> MLTEGISIQSYDGHTFGALVGSPAKAPAPVIVIAQDIFGVNAFMRETVSWLVDQGYAAVCPDLYARQAPGTALDPQDERQREQAYKLWQAFDMEAGVGDLEAAIRYARHQPYSNGKVGLVG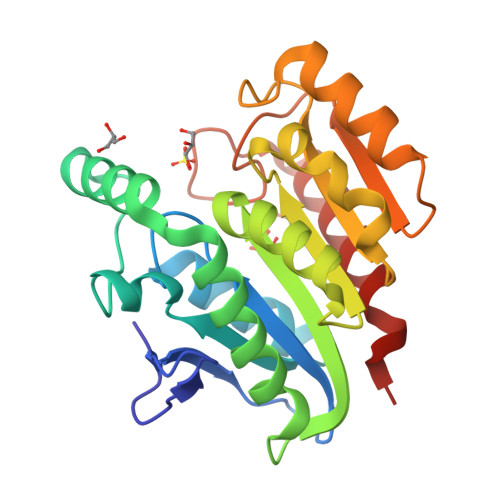YSLGGALAFLVAAKGYVDRAVGYYGVGLEKQLNKVPEVKHPALFHMGGQDHFVPAPSRQLITEGFGANPLLQVHWYEEAGHSFARTSSSGYVASAAALANERTLDFLAPLQSKKP> AKCVSYGVAQIKAPALHSQGYTGSNVKVAILDTGIDSSHPDLNVAGGASFVPSETNPFQDNSSGGTHIAGTVLAVAPSASLYAVKVLGADGKGQASWIINGIEWAIANNMDVINMSLGSPSGSAAVKAAVDKAVASGVVVVAAAGNSGTSGSSSTVTYPAKYPSVIAVGAVDSSNQRAPFSSVGPELDVMAPGVSICSTLPGGKYGALSGTSMASPHVAGAAALILSKHPNWTNTQVRSSLENTATKLGDSFYYGKGLINVEAAAQ

We describe the design, kinetic properties, and structures of engineered subtilisin proteases that degrade the active form of RAS by cleaving a conserved sequence in switch 2. The engineering process to develop specificity for the RAS sequence QEEYSAM involved extensive modification of the Bacillus protease, subtilisin BPN’16–24, a canonical serine protease in which the scissile peptide bond is attacked by a nucleophilic serine (S221). The nucleophilicity of S221 results from its interactions with the catalytic histidine (H64) and aspartic acid (D32) that together form a charge relay system. To generate high specificity for the RAS target sequence, the active site was modified to be dependent on a cofactor (imidazole or nitrite) and protease sub-sites were engineered to create a linkage between substrate and cofactor binding.

The two S101K mutants are denoted as RAS-specific proteases RASProtease(N) and RASProtease(I). To understand the structural basis for specificity and cofactor activation, we determined crystal structures of RASProtease(I) alone, in complex with YSAM and QEEYSAM product peptides, and with imidazole. The structures also provide insight into the structural basis for cofactor activation by both nitrite in Protease1(N) and imidazole in RASProtease(I). In both cases, a catalytic amino acid is mutated to Gly and the vacated space is occupied by a network of conserved water molecules in the absence of the cognate cofactor. Structures of RASProtease(I) without imidazole have three conserved waters (19, 81, and 122) that interact with Oδ1 and Oδ2 of D32, CO of S125, NH of G64, Oγ of S62, and Oγ of S221. When imidazole binds, these waters are displaced, the imidazole nitrogens H-bond to Oδ1 and Oδ2 of D32 and Oγ of S221, and the charge relay system is reconstituted. RAS-specific proteases have an expanded S4 site that binds numerous solvent molecules in the enlarged S4 pocket.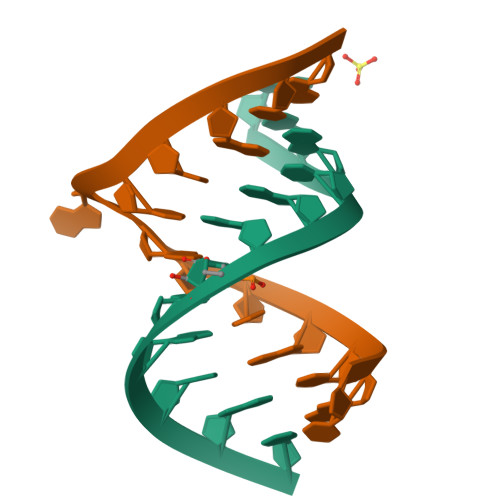> GCGCGGUAGUGC;> CGCACUAACCGCG4-[2,4-bis(oxidanylidene)-6-(trifluoromethyl)-1H-pyrimidin-3-yl]-5-methyl-2-(2-methylphenoxy)benzenecarbonitrile | C20 H14 F3 N3 O3 | 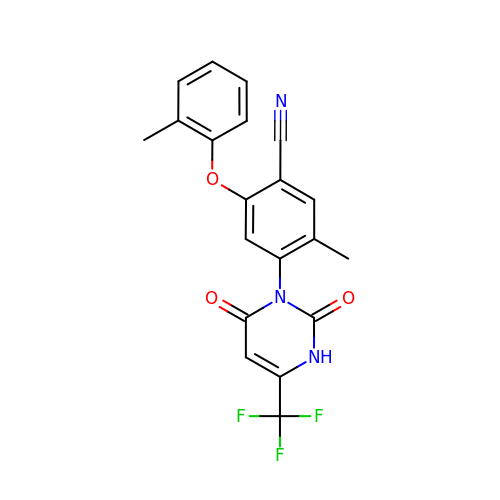XSDNYWMZDXTSBT-UHFFFAOYSA-N>MKIVLAYSGGLDTSIILKWLKETYRAEVIAFTADIGQGEEVEEAREKALRTGASKAIALDLKEEFVRDFVFPMMRAGAVYEGYYLLGTSIARPLIAKHLVRIAEEEGAEAIAHGATGKGNDQVRFELTAYALKPDIKVIAPWREWSFQGRKEMIAYAEAHGIPVPVTQEKPYSMDANLLHISYEGGVLEDPWAEPPKGMFRMTQDPEEAPDAPEYVEVEFFEGDPVAVNGERLSPAALLQRLNEIGGRHGVGRVDIVENRFVGMKSRGVYETPGGTILYHARRAVESLTLDREVLHQRDMLSPKYAELVYYGFW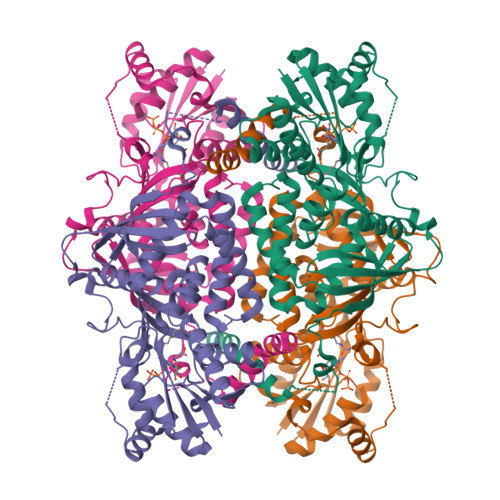YAPEREALQAYFDHVARSVTGVARLKLYKGNVYVVGRKAPKSLYRQDLVSFDEAGGYDQKDAEGFIKIQALRLRVRALVEREGHGA[4x]> DDDGEHGGRRAALVVTDPLTRTECSACHMAYPAALLPARSWTALMADLPNHFGEDASLDEASRGQIESYLVANAADSSG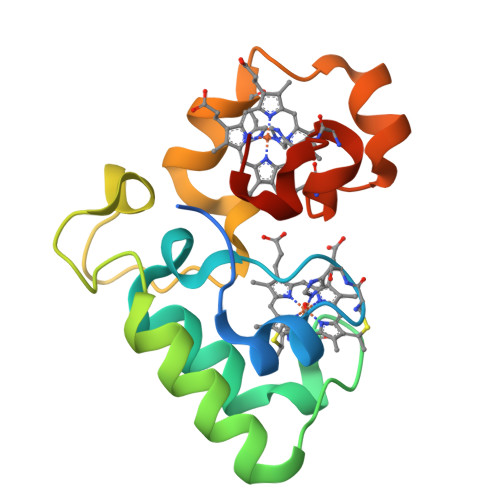AGRALRGLVQTDTPLRISELPWFKRKHADEVSPRMLEKARSMSNCAACHTGAERGLFDDD>MSLAQKLRQASSRLLGVVFELQQPFHGDLVEQIYAAATRRGYDVMLSAVAPSRAEKVAVQ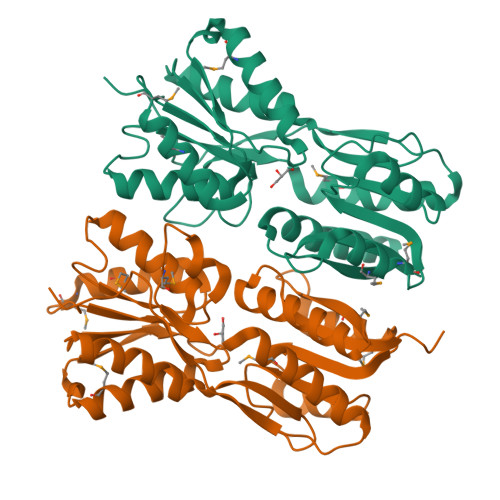ALMRERCEAAILLGTRFDTDELGALADRVPALVVARASGLPGVGAVRGDDVAGITLAVDHLTELGHRNIAHIDGADAPGGADRRAGFLAAMDRHGLSASATVVTGGTTETEGAEGMHTLLEMPTPPTAVVAFNDRCATGVLDLLVRSGRDVPADISVVGYDDSRLARIPHVQMTTISQDATHMAEAAVDGALAQISGDKAVDLVLAPHLVRRATTGPVAHREGHHHHHH[2x]>MGHHHHHHMTIPDKIKAVYEKSTCLYTSNEVEAALDRMAIKIHETLQDKNPVIICVMVGGLVPLGNLLHRLDFPLEVDYVHATRYRGDLTGGDILWKVRPSSNLAGRTVLVVDDILDGGITLAAIINEIKAMGAAEVYSAVLVDKYRKRVPNGLQKADF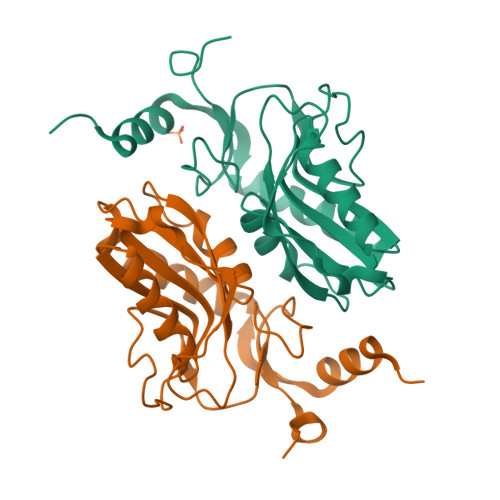VGLQVEDHYIFGYGMDYHEYLRNAPGIFIVHPDHEASK[2x]>[3x]VDFHGYARSGIGWTGSGGEQQCFQATGAQSKYRLGNECETYAELKLGQEVWKEGDKSFYFDTNVAYSVNQQNDWESTDPAFREANVQGKNLIEWLPGSTIWAGKRFYQRHDVH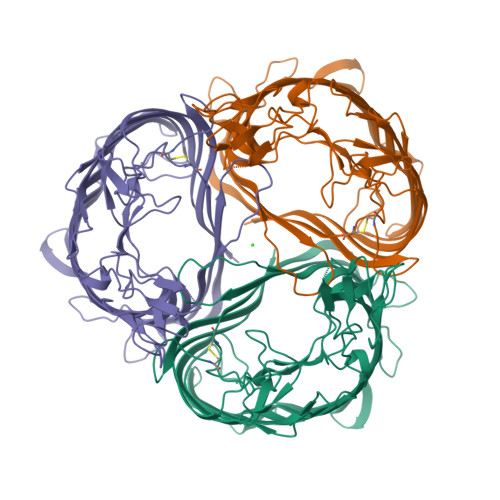MIDFYYWDISGPGAGIENIDLGFGKLSLAATRSTEAGGSYTFSSQNIYDEVKDTANDVFDVRLAGLQTNPDGVLELGVDYGRANTTDGYKLADGASKDGWMFTAEHTQSMLKGYNKFVVQYATDAMTTQGKGQARGSDGSSSFTEELSDGTKINYANKVINNNGNMWRILDHGAISLGDKWDLMYVGMYQNIDWDNNLGTEWWTVGVRPMYKWTPIMSTLLEVGYDNVKSQQTGDRNNQYKITLAQQWQAGDSIWSRPAIRIFATYAKWDEKWGYIKDGDNISRYAAATNSGISTNSRGDSDEWTFGAQMEIWW In this work, we exhaustively probe the ability of all 36 immobile HJ sequences to form DNA crystals in two different designed systems. Three separate self-assembling DNA crystal systems are described in this report: the “4 × 5” and “4 × 6” designs (collectively referred to as the 4 × N systems), and a third construct with a “scrambled” sequence variant of the 4 × 6 lattices. Self-assembly was mediated by three constituent oligonucleotides: (S1) containing four sequence repeats of either 5 or 6 bases; (S2) composed of 21 bases containing complementary regions to both (S1); and (S3) which forms the second junction crossover. The HJ serves as the fundamental component at the core of each unit, and the ultimate assembly of the full lattice is facilitated by the complementary 2-base sticky ends that tail each duplex.

The 4 × 5 system robustly crystallized with 75% of the junctions, and we obtained crystals in all but 9 of 36 sequences. Of the resulting structures, 18 exhibited P32 symmetry with average cell dimensions a = b = 68.85 Å c = 60.09 Å, with only nine retaining the original P3221 symmetry with average cell edges a = b = 68.17 Å c = 60.60 Å. Although the cell parameters between the two symmetries were virtually indistinguishable, the differences between the periodicity of the lattices is dramatic, with vastly different cavity sizes. Pos1 and 2 were readily observable in the electron density maps at either one or both of these conserved sites in a significant number of the structures, with no apparent respect to motif or symmetry. However, in the majority of the crystal structures reported here, the cacodylate anion indeed fits best into the electron density map of our X-ray structures, due to the presence of sodium cacodylate in the crystallization solution.

> GAGCAGACCAG;> ACTCCACTCA;> CTAGT;> TCTGAGTGGGGTCTGC>[2x]GSHMAAVDLATHPGHLARRLQQAHYLLWNTMVSEETTSPQYAVLNALVAEPGLDQRTVGERVGLDRSTIAEVVSRLGRRGLLDKVRDPQDGRRSLLRLTDEGLRVHRRLGVRIARMNQ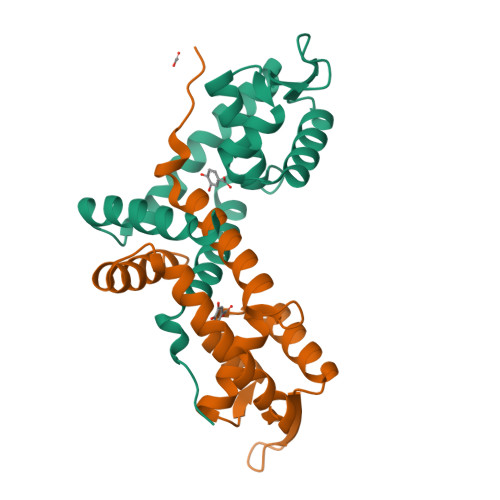VFLAPLAADEQAVFFDLIRRVADAAEGLRNPAEPAVAPG>MGALRIDSHQHFWRYRAADYPWIGAGMGVLARDYLPDALHPLMHAQALGASIAVQARAGRDETAFLLELACDEARIAAVVGWEDLRAPQLAERVAEWRGTKLRGFRHQLQDEADVRAFVDDADFARGVAWLQANDYVYDVLVFERQLPDVQAFCARHDAHWLVLDHAGKP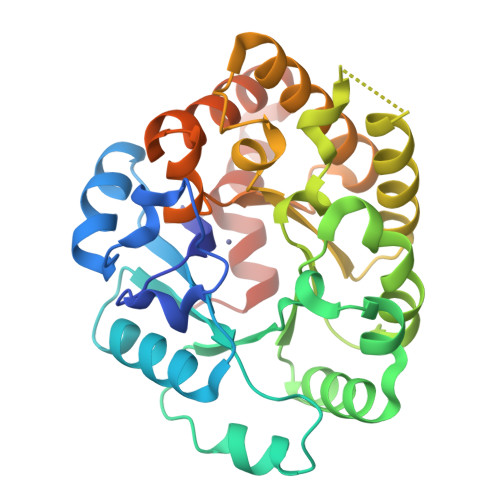ALAEFDRDDTALARWRAALRELAALPHVVCKLSGLVTEADWRRGLRASDLRHIEQCLDAALDAFGPQRLMFGSDWPVCLLAASYDEVASLVERWAESRLSAAERSALWGGTAARCYALPEPADARLAENLYFQ[2x]In this paper, we report the crystallization and the crystal structure of a 43 kDa recombinant thermostable lipase isolated from Bacillus sp. L2. The structure possesses the known fold of the a/b hydrolase family, and contains both a calcium ion and a zinc ion. Lipases catalyze both the hydrolysis of triglycerides to glycerols and free fatty acids over an oil-water interface, and also the hydrolysis and transesterification of other esters as well as the synthesis of esters and exhibiting enantioselective properties. Bacterial lipases are members of the structural superfamily of α/β hydrolases whose enzymic activity results from the catalytic triad Ser-His-Asp, similar to that found in serine proteinases.

Crystallization of L2 lipase was done using a counter diffusion method in collaboration with JAXA (Japanese Aerospace Exploration Agency) under the JAXA-UPM Protein Crystal Growth (PCG) #1 Flight 1 program. The best Shape 2 L2 lipase crystal was diffracted at high resolution (1.5 Å) and belongs to the orthorhombic space group P212121, with unit-cell parameters a = 72.0, b = 81.8, c = 83.4 Å, α = β = γ = 90°. The core structure L2 lipase is made of a seven-stranded parallel sheet that is surrounded by a number of alpha helices; namely alpha helices 1 and 13 on one side, and alpha helices 2, 4, 5, 9,10, 11 and 12 on the opposite site of the structure. Based on the structural alignment of L2 lipase with other structurally-known lipases, the Ser113, Asp317 and His358 were assigned as the catalytic triad. The catalytic serine residue (Ser113) lies in the generously allowed region and situated on the nucleophilic elbow between strand b5 and helix a4 deep within the core structure. L2 lipase contains the Ala-Xaa-Ser-Xaa-Gly pentapeptide, which is the conserved form in Bacillus spp. The pentapeptide of L2 lipase consisted of Ala-His-Ser-Gln-Gly. The lid of the L2 lipase structure is formed by helix α6. In the L2 lipase structure, the Ca2+ is coordinated in an octahedral environment via Gly286 O, Glu360 O Asp365 O, Pro366 O and two water molecules. The Zn2+ is coordinated in a tetrahedral environment by two histidine N12 atoms (His81 and His87) located in helix α3, and two aspartate O atoms (Asp61 and Asp238). The Zn2+ is approximately 19 Å away from the catalytic serine residue, and is thus unlikely to participate in catalysis.

> HHHHHHASLRANDAPIVLLHGFTGWGREEMFGFKYWGGVRGDIEQWLNDNGYRTYTLAVGPLSSNWDRACEAYAQLVGGTVDYGAAHAAKHGHARFGRTYPGLLPELKRGGRIHIIAHSQGGQTARMLVSLLENGSQEEREYAKAHNVSLSPLFEGGHHFVLSVTTIATPHDGTTLVNMVDFTDRFFDLQKAVLEAAAVASNVPYTSQVYDFKLDQWGLRRQPGESFDHYFERLKRSPVWTSTDTARYDLSVSGAEKLNQWVQASPNTYYLSFSTERTYRGALTGNHYPELGMNAFSAVVCAPFLGSYRNPTLGIDDRWLENDGIVNTVSMNGPKRGSSDRIVPYDGTLKKGVWNDMGTYNVDHLEIIGVDPNPSFDIRAFYLRLAEQLASLLP>[2x]MAHHHHHHVDDDDKMASSSNYNTYMQYLNPPPYADHGANQLIPADQLSNQQGITPNYVGDLNLD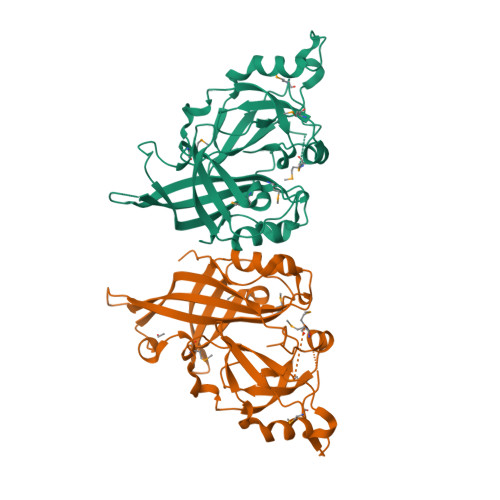DQFKGNVCHAFTLEAIIDISAYNERTVKGVPAWLPLGIMSNFEYPLAHTVAALLTGSYTITQFTHNGQKFVRVNRLGTGIPAHPLRMLREGNQAFIQNMVIPRNFSTNQFTYNLTNLVLSVQKLPDDAWRPSKDKLIGNTMHPAVSIHPNLPPIVLPTVKKQAYRQHKNPNNGPLLAISGILHQLRVEKVPEKTSLFRISLPADMFSVKEGMMKKRGENSPVVYFQAPENFPLNGFNNRQVVLAYANPTLSAV>MGSSIK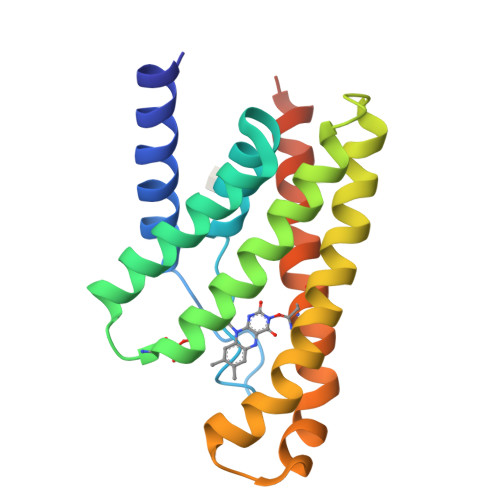KISFVGIFSALATLVMFLEFPIFPQASFLKYDPSEIPALIVSFLLGPGVGMFVVLVKDILFFLMKSGDPVGIAMNAVLGMSFVGIAGLIYHRNKSRATAIKGMIVATLFATAFALGLNALIVPLYFEAPFELYLKFFPFILAFNLVKFGIDSVVTFFVYKKVSSILKLSNSLVPR[2x]>MSVLLSGTVTAKNEQYVYFDASKGDLDEILVSVGDKVS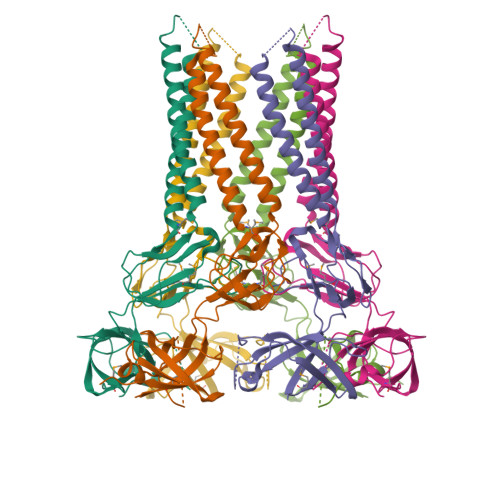EGQALVKYSSSEAQAAYDSASRAVARADRHINELNQARNEAASAPAPQLPAPVGGEDATVQSPTPVAGNSVASIDAQLGDARDARADAAAQLSKAQSQLDAMTVLSTLEGTVVEVNSNVSKSPTGASQVMVHIVSNENLQVKGELSEYNLANLSVGQEVSFTSKVYPDKKWTGKLSYISDYPKNNGEAASPAAGNNTGSKYPYTIDVTGEVGDLKQGFSVNMEVKSKTKHHHHHH[3x]Indanomycin is an antibiotic from the pyrroloketo­indane family which is known to act as an effective ionophoric agent against Gram-positive bacteria. IdmH is a homodimer, with the individual protomers consisting of an α+β barrel. Each protomer contains a deep hydrophobic pocket which is proposed to constitute the active site of the enzyme.

To improve crystallization, a number of variants were produced to reduce the surface entropy or to truncate predicted surface loops (Roy et al., 2010). One variant, containing a deletion of residues 99–107, resulted in large, easily reproducible crystals in the cubic space group F23 [Supplementary Fig. S5(b)] from new crystallization conditions. Here, the crystal structure of a selenomethionine-labelled truncated form of IdmH (IdmH-Δ99–107) was solved using single-wavelength anomalous dispersion (SAD) phasing. The asymmetric unit comprises one copy of the IdmH-Δ99–107 dimer with the entire polypeptide chain successfully modelled into density, except for the N- and C-terminal regions. Both the selenomethionine-labelled protein structure and the isomorphous native structure of IdmH-Δ99–107 were modelled independently, giving almost identical structures that superpose with an r.m.s.d. of 0.12 Å over 257 amino acids.

>GSHMAHQPSDTIAGLYEAFNSGDLETLRELIAPDAVIHLPGTAGDAEHPPGTPRDREGWLGVWQFTQAFFPDMTATVQDIVQTGDLVATRCVARGTHSGRPFEMTMLNMSRVRDGRIVEHWTISDNVTMLAQLGVKASL[2x]Human adenoviruses (HAdV) are double stranded DNA viruses with non-enveloped icosahedral capsids. Adenoviruses have a conserved icosahedral capsid structure, consisting of three major proteins: hexon, penton base and fiber proteins. Hexon protein, the most abundant of the capsid, forms 240 trimeric capsomeres making up the facets of the icosahedron. Minor proteins, protein (p)IIIa, pIX, pVIII and pVI, play a structural role in the capsid alongside the major proteins.

HAdV-D10 has low seroprevalence across human populations making it a compelling candidate for development as a therapeutic vector. Single particle analysis using icosahedral symmetry led to the calculation of a capsid reconstruction at 3.3 Å resolution using a total of 5,524 capsid particles. The structure of the HAdV-D10 capsid is largely similar to previously published mastadenovirus structures with global pseudo-icosahedral symmetry with a T=25 capsid. The sharply resolved map supported the assembly of models for hexon, penton, pIX, pVIII, pIIIa and pVI. The full length, 949 amino acid, atomic model could be built for hexon protein. The overall architecture of hexon protein closely matches HAdV-C5 and HAdV-D26 with root mean square deviations (RSMD) of 1.158 Å and 2.448 Å respectively. A copy of the penton base is found at each of the twelve vertices. The penton base (coloured in cyan in [Fig fig1]) is highly conserved compared to HAdV-C5 (RMSD 0.762) and HAdV-D26 (RMSD 0.492), and similarly is well resolved except for residues 297-324 which correspond to the loop containing the integrin binding RGD motif ([Fig fig1] and [Fig fig1]). The flexible loop contains an RGD motif that engages with host cellular integrins and corresponds to residues 299-324 in HAdV-D10. In conclusion, we have combined the first whole capsid structure of the HAdV-D10 capsid at 3.3 Å ([Fig fig1] and S1) with the first transcriptomic investigations ([Fig fig4]) of the same virus, revealing unique features and insights into its biology.

>MEDINFASLAPRHGTRPFMGTWNEIGTSQLNGGAFNWSSVWSGLKNFGSTLRTYGNKAWNSSTGQLLREKLKDQNFQQKVVDGLASGINGVVDIANQAVQREINSRLDPRPPTVVEMEDATLPPPKGEKRPRPDAEETILQVDEPPSYEEAVKAGMPTTRIIAPLATGVMKPATLDLPPPPAPAPPKATPVVQAPPVATAVRRVPARRQAQNWQSTLHSIVGLGVKSLKRRRCY[8x];>[12x]MMPQWAYMHIAGQDASEYLSPGLVQFARATDTYFSLGNKFRNPTVAPTHDVTTDRSQRLTLRFVPVDREDTTYSYKARFTLAVGDNRVLDMASTYFDIRGVLDRGPSFKPYSGTAYNSLAPKSAPNPSQWTANEKQTGGQPKSVTQTFGSAPMGGSNITIEGLVIGTKEEEGNATEEIFADKTFQPEPQVGEENWQETEAFYGGRALKKDTKMKPCYGSFARPTNEKGGQAKLKLNDQGQPTKDYDIDLAFFDTPGGTPPTGSGQQEEYKADIVMYTENVNLETPDTHVVYKPGKEDESSETNLTQQSMPNRPNYIGFRDNFVGLMYYNSTGNMGVLAGQASQLNAVVDLQDRNTELSYQLLLDSLGDRTRYFSMWNSAVDSYDPDVRIIENHGVEDELPNYCFPLNGTGTNSTYQGVKVKTGQDGAEETEWDKDETVARQNQIAKGNVYAMEINLQANLWKSFLYSNVALYLPDSYKYTPANVTLPANTNTYEYMNGRVVAPSLVDAYINIGARWSLDPMDNVNPFNHHRNAGLRYRSMLLGNGRYVPFHIQVPQKFFAIKNLLLLPGSYTYEWNFRKDVNMILQSSLGNDLRVDGASVRFDSVNLYATFFPMAHNTASTLEAMLRNDTNDQSFNDYLSAANMLYPIPAKATNVPISIPSRNWAAFRGWSFTRLKTKETPSLGSGFDPYFVYSGSIPYLDGTFYLNHTFKKVSIMFDSSVSWPGNDRLLTPNEFEIKRSVDGEGYNVAQCNMTKDWFLVQMLSHYNIGYQGFHVPEGYKDRMYSFFRNFQPMSRQVVDEINYKDYKAVTLPFQHNNSGFTGYLAPTMRQGQPYPANFPYPLIGQTAVPSVTQKKFLCDRVMWRIPFSSNFMSMGALTDLGQNMLYANSAHALDMTFEVDPMDEPTLLYLLFEVFDVVRVHQPHRGVIEAVYLRTPFSAGN;> MRRAVVSSSPPPSYESVMAQATLEVPFVPPRYMAPTEGRNSIRYSELAPQYDTTRVYLVDNKSADIASLNYQNDHSNFLTTVVQNNDFTPAEASTQTINFDERSRWGGDLKTILHTNMPNVNEYMFTSKFKARVMVARKHPEGVVETDLSQDKLEYEWFEFTLPEGNFSETMTIDLMNNAILENYLQVGRQNGVLESDIGVKFDSRNFKLGWDPVTKLVMPGVYTYEAFHPDVVLLPGCGVDFTESRLSNLLGIRKKQPFQEGFRIMYEDLEGGNIPALLDVPKYLESKKKVEDETKNAAAATADTTTRGDTFATPAQETAADKKVEVLPIEKDESGRSYNLIQGTHDTLYRSWYLSYTYGDPEKGVQSWTLLTTPDVTCGAEQVYWSLPDLMQDPVTFRSTQQVSNYPVVGAELMPFRAKSFYNDLAVYSQLIRSYTSLTHVFNRFPDNQILCRPPAPTITTVSENVPALTDHGTLPLRSSIRGVQRVTVTDARRRTCPYVYKALGIVAPRVLSSRTF;> MQQAPDPAIRAALQSQPSGIASDDWEAAMQRIMALTTRNPESFRQQPQANRLSAILEAVVPSRTNPTHEKVLAIVNALAENKAIRPDEAGLVYNALLERVGRYNSTNVQSNLDRLVTDVREAVAQRERFKNEGLGSLVALNAFLATQPANVPRGQDDYTNFISALRLMVTEVPQSEVYQSGPDYFFQTSRQGLQTVNLSQAFKNLRGLWGVQAPVGDRSTVSSLLTPNSRLLLLLIAPFTDSGSVNRNSYLGHLLTLYREAIGQAQVDEQTFQEITSVSRALGQNDTDSLRATLNFLLTNRQQKIPAQYALSAEEERILRYVQQSVGLFLMQEGATPSAALDMTARNMEPSMYAANRPFINKLMDYLHRAAVMNTDYFTNAILNPHWLPPPGFYTGEYDMPDPNDGFLWDDVDSVVFSPTFQKRQEAPPSEGAVGRSPFPSLGSLHSLPGSVNSGRVSRPRLLGEDEYLNDSLLQPPRAKNAMANNGIESLVDKLNRWKTYAQDHRDAPAPRRQRHDRQRGLVWDDEDSADDSSVLDLGGSGGVNPFAHLQPKLGRRMF;>[2x]MSKEIPTPYMWSYQPQMGLAAGASQDYSTRMNWLSAGPSMISRVNGVRNHRNQILLEQAAVTSTPRAKLNPRNWPSTLVYQEIPGPTTVLLPRDALAEVRMTNSGVQLAGGASRCPLRPQSGIKTLVIRGRGTQLNDELVSSSIGLRPDGVFQLAGAGRSSFTPNQAYLTLQSSSSEPRSGGIGTLQFVEEFVPSVYFNPFSGSPGLYPDEFIPNFDAVREAVDGYD;>MNGTGGAFEGGLFSPYLTTRLPGWAGVRQNVMGSTVDGRPVLPANSSTMTYATVGSSSLDSTAAAAAAAAAMTATRLASSYMPSSGSSPSVPSSIIAEEKLLALLAELEALSRQLAALTQQVSELREQQQQQNK[4x]> GGAGGGGAAAUUCUA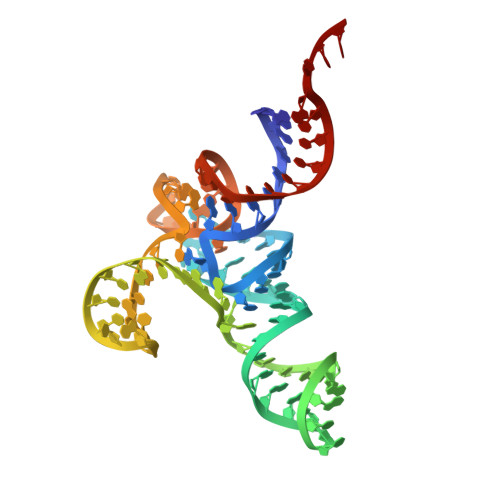UCUGGUGAUAGACGGGAACUCUAAAUUCCUUGAAAUGCCUCGCCGCAUUGGGUUCGAUUCCCUUCCCCUCCGCCA> MTTTERPDLAWLDEVTMTQLERNPYEVYERLRAEAPLAFVPVLGSYVASTAEVCREVATSPDFEAVITPAGGRTFGHPAIIGVNGDIHADLRSMVEPALQPAEVDRWIDDLVRPIARRYLERFENDGHAELVAQYCEPVSVRSLGDLLGLQEVDSDKLREWFAKLNRSHTNAAVDENGEFANPEGFAEGDQAKAEIRAVVDPLIDKWIEHPDDSAISHWLHDGMPPGQTRDREYIYPTIYVYLLGAMQEPGHGMASTLVGLFSRPEQLEEVVDDPTLIPRAIAEGLRWTSPIWSATARISTKPVTIAGVDLPAGTPVMLSYGSANHDTGKYEAPSQYDLHRPPLPHLAFGAGNHACAGIYFANHVMRIALEELFEAIPNLERDTREGVEFWGWGFRGPTSLHVTWEV

GcoA belongs to the CYP255A family of cytochrome P450 enzymes. Our recent characterization of a two-component P450 enzyme system consisting of a reductase, GcoB, and a P450 oxidase, GcoA, demonstrated that it demethylates diverse aromatic compounds, including guaiacol (which can be derived from coniferyl alcohol and represents the aromatic functionality of G-lignin that must undergo demethylation), guaethol, anisole (methoxybenzene), 2-methylanisole, and 3-methoxycatechol (3MC) with similar or greater efficiency than other O-aryl-demethylases described in the literature. However, GcoAB shows poor reactivity toward syringol, which can be derived from sinapyl alcohol via high-temperature reactions and represents the aromatic functionality of S-lignin that must undergo O-demethylation for further catabolism via ring-opening dioxygenases. In the present study, we hypothesized that substitution of GcoA-F169, which has the closest interaction with the bound substrate, may relax the specificity of the enzyme sufficiently to permit the O-demethylation of S-lignin type substrates.

The closest contact is with GcoA-F169, which forms a hydrophobic interaction with the C6 carbon on the aromatic ring of guaiacol. Each protein variant also crystallized successfully with guaiacol and the structures showed that the orientation of the bound ligand remained consistent with that of the WT enzyme. Furthermore, comparison of the surrounding active site architecture confirmed no significant deviation from the WT. Thus, the GcoA-F169A mutant, which showed enhanced turnover on guaiacol and syringol, is closer to the CYP255A consensus protein than the WT. It is interesting that although none of the GcoA homologs in our analyses exhibits a histidine at position 169, the GcoA-F169H mutant was stable and showed the highest specific activity on guaiacol.>[5x]GSHMGGVEVLEVKTGVDAITEVECFLNPEMGDPDENLRGFSLKLSAENDFSSDSPERKMLPCYSTARIPLPNLNEDLTCGNLLMWEAVTVQTEVIGITSMLNLHAGSQKVHEHGGGKPIQGSNFHFFAVGGDPLEMQGVLMNYRTKYPDGTITPKNPTAQSQVMNTDHKAYLDKNNAYPVECWVPDPSRNENTRYFGTFTGGENVPPVLHVTNTATTVLLDEQGVGPLCKADSLYVSAADIC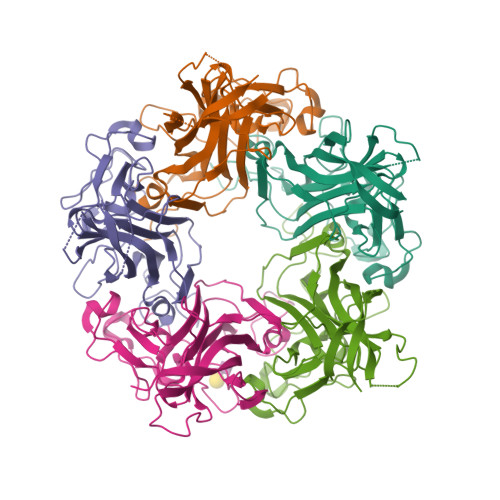GLFTNSSGTQQWRGLARYFKIRLRKRSVKNPYP>MARVLVVDDAAFMRMLLKKILTQAGHEVVGEASNGKEAVEKYKQLKPDLVTMDIVMPEMDGITAVKEIMKIDPNAKIIMITAVGQEAKVMEALKSGAKGY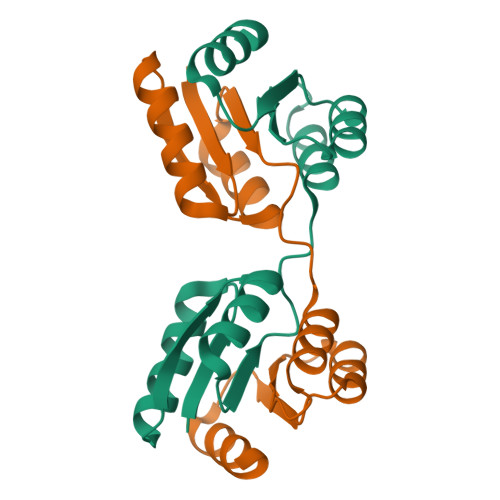IVKPFQAQKVIEEVNRVLSS[3x]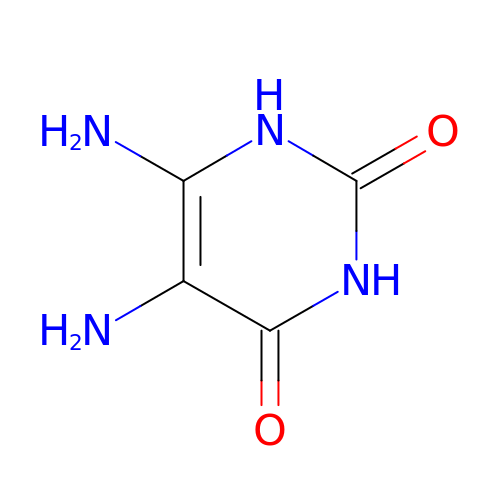5,6-DIAMINOPYRIMIDINE-2,4(1H,3H)-DIONE | C4 H6 N4 O2 | BBTNLADSUVOPPN-UHFFFAOYSA-N> MVREPATEAEAALCAVYAEVLGLDKVGADADFFALGGDSVLTLRLVHRARSAGWEISARHVFRHPVVADLAAVAQPVTEGSHHHHHH

Non-ribosomal peptide synthetases are important enzymes for the assembly of complex peptide natural products. Within these multi-modular assembly lines, condensation domains perform the central function of chain assembly, typically by forming a peptide bond between two peptidyl carrier protein (PCP)-bound substrates. To address this, we report the structure and biochemical characterization of complexes of a PCP domain bearing a stable analog of the acyl acceptor complexed to the acceptor site of a C domain from the NRPS that biosynthesizes fuscachelin in the thermophile Thermobifida fusca. The C3 domain of the didomain resembles other members of its class, comprising a pseudo-dimer of CAT domains with bridge (R2923 to T2944) and floor loop (A2843 to L2858) regions.

Given that the PCP2 and PCP3 domains of the fuscachelin NRPS are highly similar (65% sequence identity), and that PCP domains can act as both aminoacyl donors and acceptors for C domains, we rationalized that the arrangement observed in our structure is a valid model of an acceptor-PCP-bound C domain. Importantly, the residues at the interface with the C domain are conserved or highly similar. Furthermore, computational docking of the PCP3 domain onto the acceptor-PCP binding site of the C3 domain showed that it binds in an almost identical orientation to the PCP2 domain in the structure of the PCP2-C3 didomain.> GS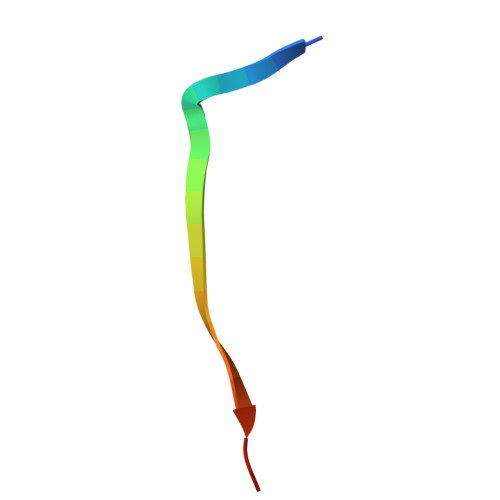FLPNSEQQKSVDAVFSSP Postsynaptic scaffold proteins such as Shank, PSD-95, Homer and SAPAP/GKAP family members establish the postsynaptic density of glutamatergic synapses through a dense network of molecular interactions. In the presence of Zn2+, the SAM-domain polymerizes into helical fibers, which may be stacked side-by-side through interhelical contacts. This enables the formation of large sheets where Shank proteins multimerize, allowing Shank proteins to serve as building blocks in deeper layers of the PSD.

On the other hand, we could not readily generate crystals from the L1800W mutant SAM domain. After one round of optimization, crystals were obtained that diffracted to 1.95 Å. Structural comparison between the crystals structures of WT and of the L1800W mutant SAM domains shows that the bulky side chain of the Trp induces a shift of the C-terminal helix, locating it further away from the Zn2+ cluster. This shift places H1835 about 2.0 Å away from the position observed for SAM WT. Furthermore, H1835 adopts a different conformation for its side chain, as well as the side chain of R1832. As a result, the Zn2+ binding site is altered or possibly destroyed. While the intrahelical contacts are partially maintained in the L1800W mutant, the interhelical contacts are completely lost as no neighboring molecule is observed at the appropriate position in the crystal. As a result, Zn2+ affinity is reduced to the effect that no Zn2+ is found in the mutant protein, whereas WT SAM domain keeps partially attached to its bound Zn2+ during the purification and crystallization procedure. The p.L1800W variant severely delays the kinetics of Zn2+-dependent polymerization of the Shank2-SAM domain.

>[6x]TKPVHLWTKPDVADWLESLNWGEHKEAFMDNEIDGSHLPNLQKEDLIDLGVTRVGHRMNIERALKQLLDR> MYGSKTFIKYVSGIPDYFKQSFPEGFTWERTTTYEDGGFLTA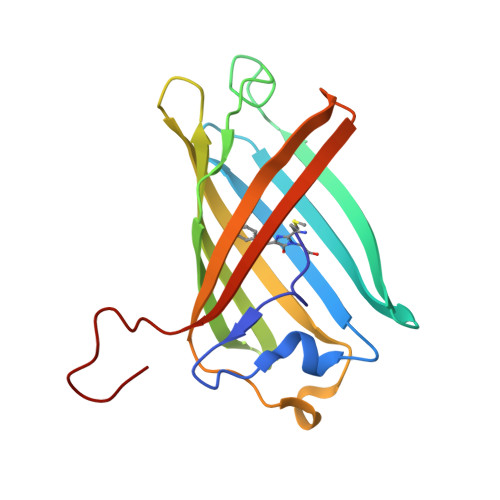HQDTSLDGDCLVYKVKILGNNFPADGPVMQNKAGRWEPATEIVYEVDGVLRGQVLMALKCPGGRHLTCHLHTTYRSKKPASALKMPGFHFEDHRIEIMEEVEKGKCYKQYEAAVGRYCDAAPSKLGHN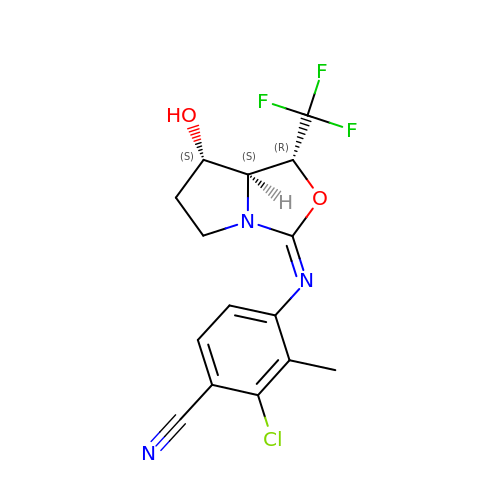2-chloro-4-{[(1R,3Z,7S,7aS)-7-hydroxy-1-(trifluoromethyl)tetrahydro-1H-pyrrolo[1,2-c][1,3]oxazol-3-ylidene]amino}-3-methylbenzonitrile | C15 H13 Cl F3 N3 O2 | KALFKWQLCWAXJO-RNSKTZJQSA-N2,3-DI-O-PHYTANLY-3-SN-GLYCERO-1-PHOSPHORYL-3'-SN-GLYCEROL-1'-PHOSPHATE 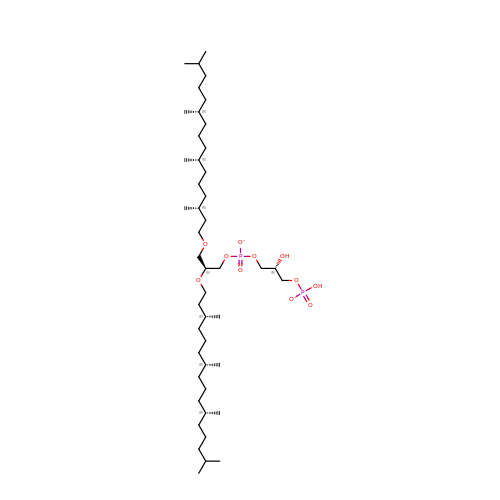| C46 H94 O11 P2 | TZXJQSKPTCRGCA-VZSPAKCESA-L>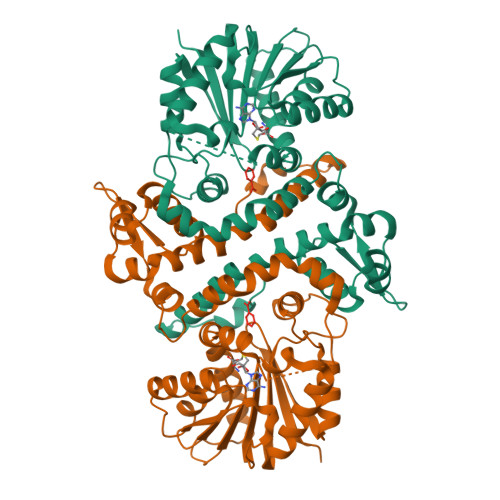[2x]MVTPEGNVSLVDESLLVGVTDEDRAVRSAHQFYERLIGLWAPAVMEAAHELGVFAALAEAPADSGELARRLDCDARAMRVLLDALYAYDVIDRIHDTNGFRYLLSAEARECLLPGTLFSLVGKFMHDINVAWPAWRNLAEVVRHGARDTSGAESPNGIAQEDYESLVGGINFWAPPIVTTLSRKLRASGRSGDATASVLDVGCGTGLYSQLLLREFPRWTATGLDVERIATLANAQALRLGVEERFATRAGDFWRGGWGTGYDLVLFANIFHLQTPASAVRLMRHAAACLAPDGLVAVVDQIVDADREPKTPQDRFALLFAASMTNTGGGDAYTFQEYEEWFTAAGLQRIETLDTPMHRILLARRATEPSAVPEGQASENLYFQ7-AMINO-3,3A,4,5-TETRAHYDRO-8H-2-OXA-5,6,8,9B-TETRAAZA-CYCLOPENTA[A]NAPHTHALENE-1,9-DIONE | C8 H9 N5 O3 | 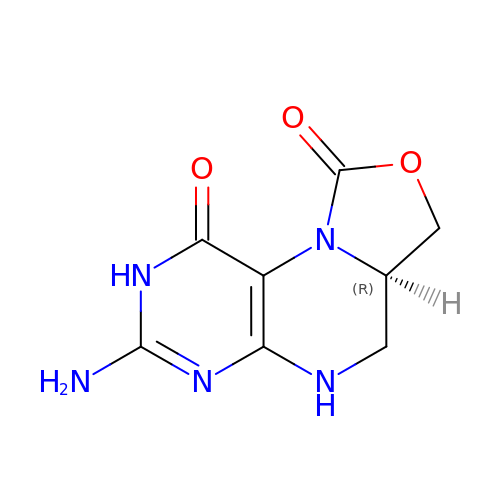XAZOBOCYEGBXHD-GSVOUGTGSA-N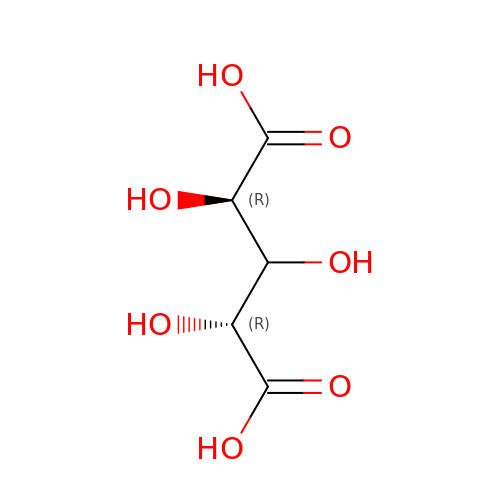L-arabinaric acid | C5 H8 O7 | NPTTZSYLTYJCPR-PWNYCUMCSA-N N-(N-FORMYLGLYCYL)-5-O-PHOSPHONO-BETA-D-RIBOFURANOSYLAMINE | C8 H15 N2 O9 P | 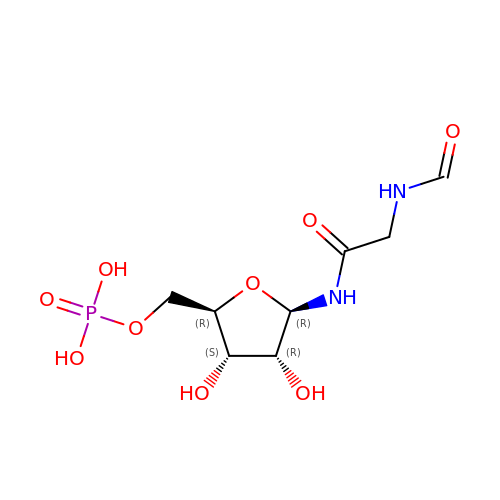VDXLUNDMVKSKHO-XVFCMESISA-N> MDHNEGGYSHHQIEGQEGQQQQAPVGGGGEDIFQVLENITQVQNEKLKRCQEFKEQENIPRQYIENSPKEELVLEHVIQFKRQFQYQLYYEDKRDLFLYPKNECDVYKFICTTIRPTKLGFLELYDYQQCSKYLSEFVQYEELDPPNEFPLVIPSPTNVAVWQKGDCFDMSILLCSLLIGVGYDAYCVYGKAPREITTRNESLMECLFLEKGKYIEENDKKPKQTLEQNENALLKKPIAHSKWDQTQETKAREAEEEKRRIALTINDDEPDELLEDPYQGQRVHCWVLLRSGKRDVQQNIFIEPSTGRMYSPSTCPYECVDAVFNNLNFWINMKPECEVKNLNFEEMDSSLNWEYVMLDTLLFNKGNGNDEEGNENIDDPLNKQAQRDPEQEQLQDIAQLLDMPPPWPPKIYIDKEKFLMGTPLGEGTVYYNKVKVDNYAPYSQPDGLVQKITIFQDYKRLKVKEYRYFYKHRSDKLSIRRRYPFEFKTIEEYEPQKYENKTIPQALQQWRQVIQIDRHLRIIKYYHNRNHDGLIERVEQIGEKTMMFYQNRDDRVIYRSIRFDNKRAPSSQNNDKVFQDNHVGDVQITKMTQKFEKNPHYPANEQIQKMVIDLIKDKVIVYYHMNDGEITPIVKIYPRDSMHGFAKLNEPGGDNKIDDPLVQLENTKMVNLEKDCLNQLKQQEKIARDDEKTIREGEIRLEKTLYDKARDRFKESSKKNDDDLAKDAAASDYLYPYLEKRKLLGVSEINAQVAMEIKNEVMQKLKERLLSRAEIIQRRLEEQRQVLEQKEAQVAKRQEIDPKQEEEIRDINFKIDILEQRALRFESMALQ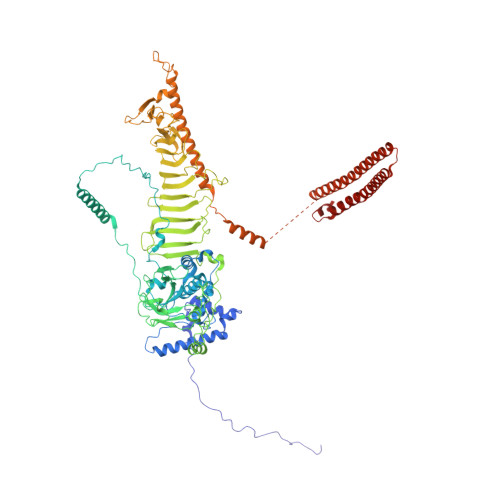KYEEMDNRLNKDARLAALHRK>MSQFFFNQRTHLVSDVIDGAIIASPWNNLARLESDPAIRIVVRRDLNKNNVAVISGGGSGHEPAHVGFIGKGMLTAAVCGDVFASPSVDAVLTAIQAVTGEAGCLLIVKNYTGDRLNFGLAAEKARRLGYNVEMLIVGDDISLPDNKHPRGIAGTILVHKIAGYFAERGYNLATVLREAQYAASNTFSLGVALSSCHLPQETDAAPRHHPGHAELGMGIHGEPGASVIDTQNSAQVVNLMVDKLLAALPETGRLAVMINNLGGVSVAEMAIITRELASSPLHSRIDWLIGPASLVTALDMKGFSLTAIVLEESIEKALLTEVETSNWPTPVPPREITCVVSSHASARVEFQPSANALVAGIVELVTATLSDLETHLNALDAKVGDGDTGSTFAAAAREIASLLHRQQLPLNNLATLFALIGERLTVVMGGSSGVLMSIFFTAAGQKLEQGANVVEALNTGLAQMKFYGGADEGDRTMIDALQPALTSLLAQPKNLQAAFDAAQAGAERTCLSSKANAGRASYLSSESLLGNMDPGAQRLAMVFKA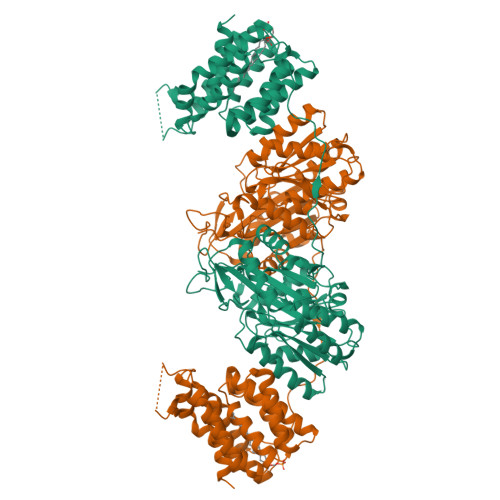LAESELG[2x]> EELQKSIGHKPEPTDEEWELIKTVTEAHVATNAQGSHWKQKRKFLPEDIGQAPIVNAPEGGKVDLEAFSHFTKIITPAITRVVDFAKKLPMFCELPCEDQIILLKGCCMEIMSLRAAVRYDPESETLTLNGEMAVTRGQLKNGGLGVVSDAIFDLGMSLSSFNLDDTEVALLQAVLLMSSDRPGLACVERIEKYQDSFLLAFEHYINYRKHHVTHFWPKLLMKVTDLRMIGACH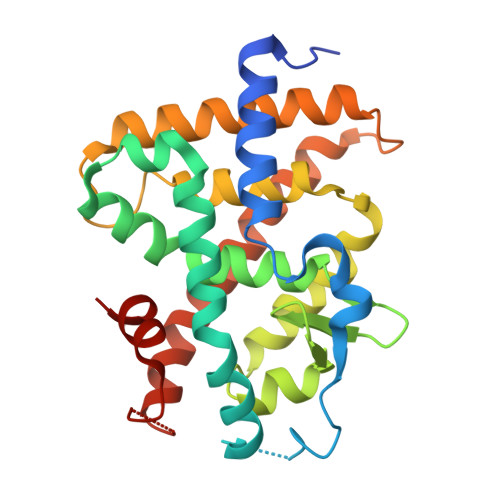ASRFLHMKVECPTELFPPLFLEVFED HORMADs were named after the first proteins in this family to be discovered in budding yeast: Hop1, Rev7, and Mad2 and meiotic HORMADs are essential to organize meiotic chromosomes for the meiosis-specific events of homolog pairing, synapsis, and recombination. Meiotic HORMAD proteins have a characteristic N-terminal HORMA domain that allows HORMADs to adopt two different conformations: a closed conformation and an open/unlocked conformation. In the closed conformation, a peptide on a binding partner called the “closure motif” binds the core of the HORMAD’s HORMA domain. This interaction is stabilized by a C-terminal region of the HORMA domain called the safety belt, which wraps around the HORMAD to lock the binding partner’s closure motif against the HORMA domain core.

Using CRISPR/Cas9 gene editing, we made a corresponding missense mutation to the htp-3H96Y allele in him-3, where arginine 93 was replaced with a tyrosine (him-3R93Y). While the closure motif for HTP-3 is unknown, HIM-3 is known to bind closure motifs found within the C-terminal tail of HTP-3. We cloned and expressed wildtype HIM-3 and HIM-3R93Y in E. coli, purified each protein, and performed a fluorescence polarization peptide binding assay to test how well HIM-3R93Y binds a peptide encoding HTP-3 closure motif #4 in vitro. Consistent with prior work, we found that wildtype HIM-3 binds the HTP-3 closure motif with a Kd of 220 +/- 20 nM and found that it does not bind to a control peptide with a scrambled sequence. HIM-3R93Y binds to the same closure motif with an increased Kd of 690 +/- 130 nM, indicating that HIM-3R93Y binds the HTP-3 closure motif with reduced affinity compared to wildtype HIM-3. The thermal stability of HIM-3R93Y is similar to that of wild-type HIM-3, and a crystal structure of HIM-3R93Y in the closed conformation is equivalent to that of wildtype HIM-3, suggesting that reduced affinity for the closure motif for HIM-3R93Y is not due to instability of the protein or an inability to adopt the closed conformation. These results demonstrate that HIM-3R93Y binds the HTP-3 closure motif less readily than wildtype HIM-3, which would potentially limit its ability to adopt the closed conformation in vivo. Right panels show the position of residue 93 and show that the overall HORMA domain structure is not impacted upon mutation of arginine 93 to tyrosine. Similar to pch-2 single mutants, we found that there was an increase of nuclei with 5 GFP::COSA-1 foci in him-3R93Y mutants compared to wildtype controls (10%, p value = 0.0004 by two-tailed Fisher’s exact test), showing that mutation of this residue in HIM-3 causes a loss of crossover assurance. Therefore, him-3R93Y suppresses the defect in crossover assurance observed in pch-2 mutants.

> MATKEQIVEHRESEIPIASQWKATFPVDLEIEKNSEMFALRYIKCASAFILDRRGILDEKCFKTRTIDKLLVTAFQSSVPAAKRVSSTFDGLYDAIQQGYLREFAIVFYKKPNEEDINEVFAFRFAYGDEGEIFVSLNNGIDTNESSQELLQAKFVDTDNTKQMFASTIKKLHRCIKKMEPLPQGSDASFRVSYTEKAPKDYTPEGYLLSPMFYTLNQDIRKASIGIVCGGHHKIQMLAASQYLKQDFDLDKTTTLNPNMSIMANQSKRKGRISRDSPYGLSQGITKKNKD>PTTKVKLECNPTARIYRKHFLGKEHFNYYSLDTALGHLVFSLKYDVIGDQEHLRLLLRTKCRTYHDVIPISCLTEFPNVVQMAKLVCEDVNVDRFYPVLYPKASRLIVTFDEHVISNNFKFGVIYQKLGATSEEELFSTNEESPAFVEFLEFLGQKVKLQDFKGFRGGLDVTHGQTGTESVYCNFRNKEIMFHVSTKLPYTE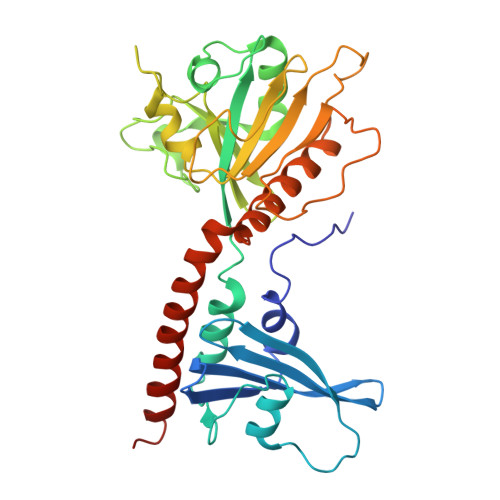GDAQQLQRKRHIGNDIVAVVFQDENTPFVPDMIASNFLHAYVVVQAEGGGPDGPLYKVSVTARDDVPFFGPPLPDPAVFRKGPEFQEFLLTKLINAEYACYKAEKFAKLEERTRAALLETLYEELHIHSQSMMGLGGDE[3x];> MREYKLVVLGSGGVGKSALTVQFVQGIFVEKYDPTIEDSYRKQVEVDAQQCMLEILDTAGTEQFTAMRDLYMKNGQGFALVYSITAQSTFNDLQDLREQILRVKDTDDVPMILVGNKCDLEDERVVGKEQGQNLARQWNNCAFLESSAKSKINVNEIFYDLVRQINR While chemical methylation of an amide bond uses a strong base to generate the imidate, OphA, the precursor protein of the fungal peptide macrocycle omphalotin A, self-hypermethylates amides at pH 7 using S-adenosyl methionine (SAM) as cofactor. Omphalotin A derives from the C terminus of the OphA protein, and it is the OphA protein that methylates its own C terminus using S-adenosyl methionine (SAM). The structure of OphA reveals a complex catenane-like arrangement in which the peptide substrate is clamped with its amide nitrogen aligned for nucleophilic attack on the methyl group of SAM. Here, we report the structure of the peptide amide methyltransferase OphA including complexes with cofactor [SAM and S-adenosyl homocysteine (SAH)], cofactor analog, substrate, and product.

Y76F, R72A, R72K, and Y98A were unmethylated even after 3 days of overexpression in E. coli. Arg72 hydrogen-bonds to Tyr76 and makes a polar contact with the carbonyl at residue i+1 (the C-terminal residue, Gly411). The Tyr76-Arg72 couple is reminiscent of the Lys-Tyr couple found in short-chain dehydrogenases/reductases (SDR) enzymes, where the positive charge stabilizes the tyrosinate anion. In addition, complexes R72A-SAH and Y76F-SAH show similar active conformation of the substrate peptide. We predict that removal of the methyl group of SAM by changing to SAH would remove the “driving force” for the flipped conformation. The structures of R72A and Y76F with SAH do show the active conformation. A different conformation of Tyr98 is seen in inactive mutant complexes (Y76F-SAM, Y76F-SAH, and R72A-SAH).

> GTSTQTKAGSLTIVGTGIESIGQMTLQALSYIEAAAKVFYCVIDPATEAFILTKNKNCVDLYQYYDNGKSALNTYTQMSELMVREVRKGLDVVGVFYGHPGVFVNPSHRALAIAKSEGYRARMLPGVSAEDCLFADLCIDPSNPGCLTYEASDFLIRDRPVSIHSHLVLFQVGCVGIADFNFTGFDNNKFGVLVDRLEQEYGAEHPVVHYIAAMMPHQDPVTDKYTVAQLREPEIAKRVGGVSTFYIPPKARKASNLDIIRRLELLPAGQVPDKKARIYPANQWEPDVPEVEPYRPSDQAAIAQLADHAPPEQYQPLATSKAMSDVMTKLALDPKALADYKADHRAFAQSVPDLTPQERAALELGDSWAIRCAMKNMPSSLLDAARESGEEASQNGFPWVIVVGVIGVIG>[5x]MDLAPQMLRELQETNAALQDVRE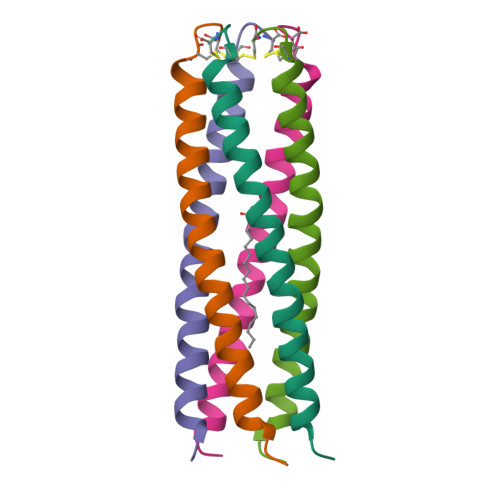LLRQQVKEITFLKNTVMECDAC>[3x]GNASSIVQTINVTGDGNVFKPSAETSSTAVPSLSLSPGMLN;>PGGVPWIAIGDETSVTSPGALRRMTSKDIPETAIINTDNSSGAVPSESALVPYNDEPLVVVTEHAIANFTKAEMALEFNREFLDKLRVLSVSPKYSDLLTYVDCYVGVSARQALNNFQKQVPVITPTRQTMYVDSIQAALKALEKWEIDLRVAQTLLPTNVPIGEVSCPMQSVVKLLDDQLPDDSLIRRYPKEAAVALAKRNGGIQWMDVSEGTVMNEAVNAVAASALAPSASAPPLEEKSKLTEQAMDLVTAAEPEIIASLVPVPAPVFAIPPKPADYNVRTLKIDEATWLRMIPKTMGTLFQIQVTDNTGTNWHFNLRGGTRVVNLDQIAPMRFVLDLGGKSYKETSWDPNGKKVGFIVFQSKIPFELWTAASQIGQATVVNYVQLYAEDSSFTAQSIIATTSLAYNYEPEQLNKTDPEMNYYLLATFIDSAAITPTNMTQPDVWDALLTMSPLSAGEVTVKGAVVSEVVPAELIGSYTPESLNASLPNDAARCMIDRASKIAEAIKIDDDAGPDEYSPNSVPIQGQLAISQLETGYGVRIFNPKGILSKIASRAMQAFIGDPSTIITQAAPVLSD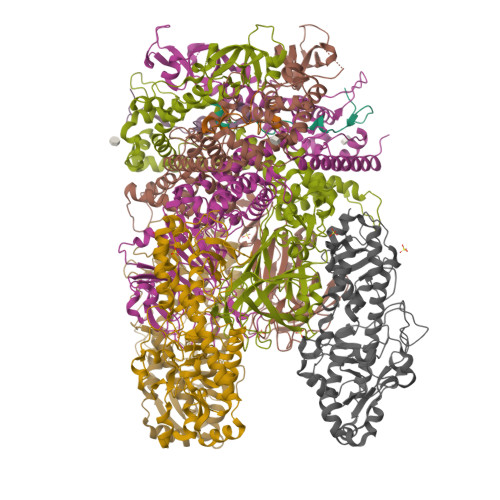KNNWIALAQGVKTSLRTKSLSAGVKTAVSKLSSSESIQNWTQGFLDKVSTHFPAPKPDCPTNGDGSEPSARRVKRDSYAGVVKRGYTR[3x];>XMEVCLPNGHQIVDLINNAFEGRVSIYSAQEGWDKTISAQPDMMVCGGAVVCMHCLGVVGSLQRKLKHLPHHRCNQQIRHQDYVDVQFADRVTAHWKRGMLSFVCQMHAMMNDVSPEDLDRVRTEGGSLVELNWLQVDPNSMFRSIHSSWTDPLQVVDDLDTKLDQYWTALNLMIDSSDLVPNFMMRDPSHAFNGVRLEGDARQTQFSRTFDSRSSLEWGVMVYDYSELEHDPSKGRAYRKELVTPARDFGHFGLSHYSRATTPILGKMPAVFSGMLTGNCKMYPFIKGTAKLKTVRKLVDSVNHAWGVEKIRYALGPGGMTGWYNRTMQQAPIVLTPAALTMFSDTTKFGDLDYPVMIGDPMILG[3x]> GSETYDFLF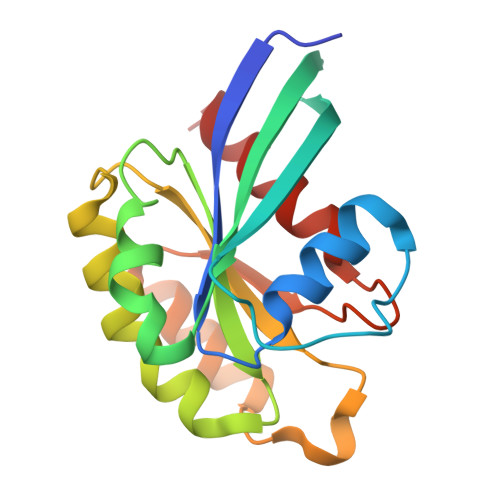KFLVIGNAGTGKSCLLHQFIEKKFKDDSNHTIGVEFGSKIINVGGKYVKLQIWDTAGLERFRSVTRSYYRGAAGALLVYDITSRETYNALTNWLTDARMLASQNIVIILCGNKKDLDADREVTFLEASRFAQENELMFLETSALTGEDVEEAFVQCARKILNK> METAVAYYK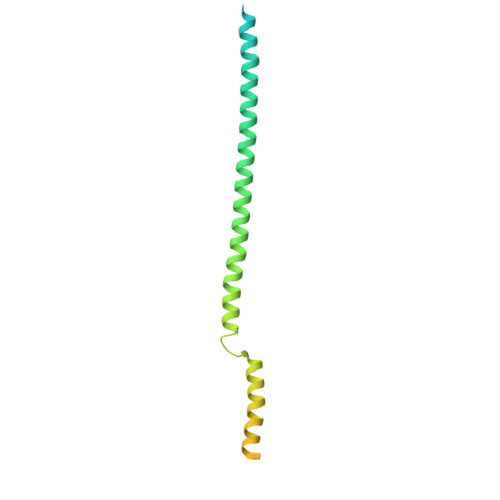DGVPYDDKGQVIITLLNGTPDGSGSGGGGGKGGSKSESSAAIHATAKWSTAQLKKTQAEQAARAKAAAEAQAKAKANRDALTQRLKDIVNEALRHNASRTPSATELAHANNAAMQAEDERLRLAKAEEKARKEAEAAEKAFQEAEQRRKEIEREKAETERQLKLAEAEEKRLAALSEEAKALEHHHHHH> RRRSGSLVYQKRRRRLLPFVSSEDPAQRLKQMGTLASALTELQMEFS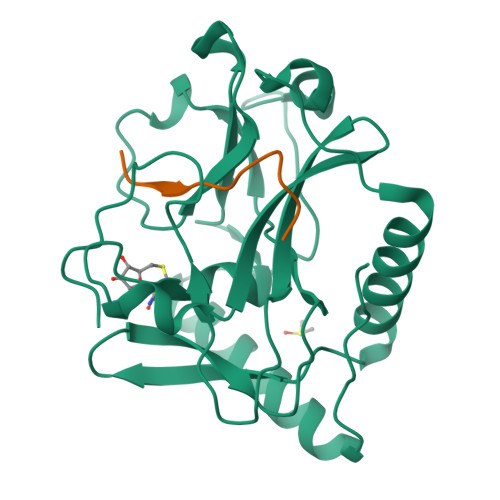DDLTYSSGMAPRSANQARFEEGGMQVLTKEDIETLEQCRAMCKRGDCPPLLVVFDSREGFTVEADGQIKDMTFIAEYTGDVDYIRNREHDDCDSMMTLLLAKDPSSSLVICPDKRGNIARFISGINNHTLDGKKKQNCKCVRYSVNGECRVFLVATRDIAKGERLYYDYNGYEHEYPTQHFV;> KQLATKAARKSAPATGGVK>SNAMPLPKSLKYGDTIGIYSPSSPVTYTSPKRFERAKSYLLQKGFHILEGSLTGRYDYYRSGSIQERAKELNALIRNPNVSCIMSTIGGMNSNSLLPYIDYDAFQNNPKIMIGYSDATALLLGIYAKTGIPTFYGPALVPSFGEFEPFVDDTYKYFLETLLHDQALPYNIKQPLFWSDEFINWEEKTKEKELRPNNWISVTNGQATGRVIGGNLNTIQGIWGSPYMPCIQEGDILFIEDSSKDAATIERSFSFLKINGVFDKVSGI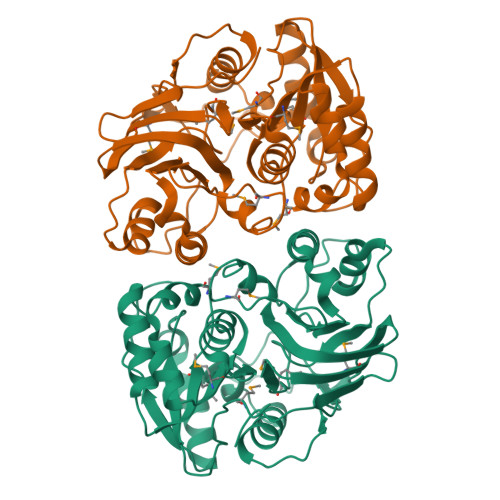ILGKHEQFDDCGTNRKPYEILLEVLQNQRIPLLADFDCCHTHPMITMPIGVQVKMDATNKTIHILEKWKI[2x]> MDLTVEPNLHSLITSTTHKWIFVGGKGGVGKTTSSCSIAIQMALSQPNKQFLLISTDPAHNLSDAFGEKFGKDARKVTGMNNLSCMEIDPSAALKDMNDMAVSRANNNGSDGQGDDLGSLLQGGALADLTGSIPGIDEALSFMEVMKHIKRQEQGEGETFDTVIFDTAPTGHTLRFLQLPNTLSKLLEKFGEITNKLGPMLNSFMGAGNVDISGKLNELKANVETIRQQFTDPDLTTFVCVCISEFLSLYETERLIQELISYDMDVNSIIVNQLLFAENDQEHNCKRCQARWKMQKKYLDQIDELYEDFHVVKMPLCAGEIRGLNNLTKFSQFLNKEYNP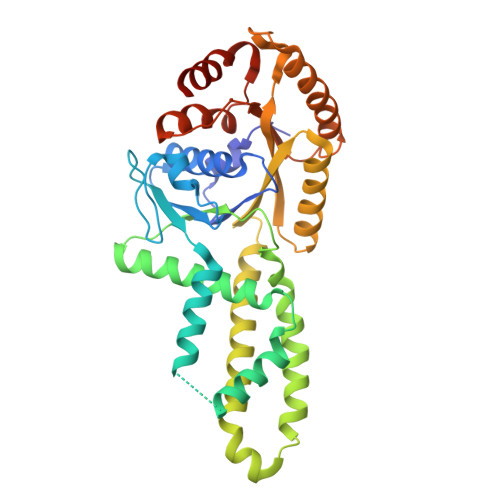ITDGKVIYELEDKELEHHHHHH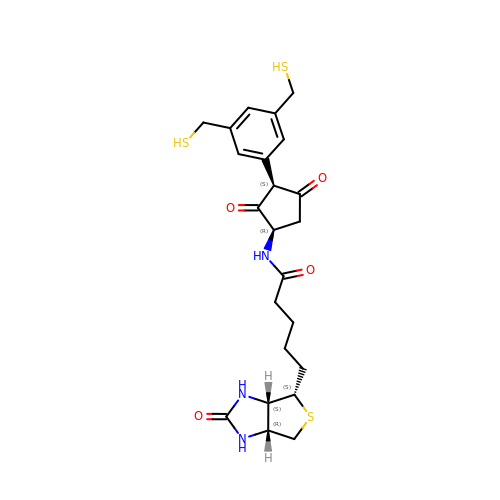5-[(3~{a}~{S},4~{S},6~{a}~{R})-2-oxidanylidene-1,3,3~{a},4,6,6~{a}-hexahydrothieno[3,4-d]imidazol-4-yl]-~{N}-[(1~{R},3~{S})-3-[3,5-bis(sulfanylmethyl)phenyl]-2,4-bis(oxidanylidene)cyclopentyl]pentanamide | C23 H29 N3 O4 S3 | UYYZXEJGUBQKBA-JSCGBJRHSA-N>[4x]MASQTITVGPWGGPGGNEWDDGSYTGIRIIELSYKEAIGSFSVIYDLNGEPFSGSKHTSKLPYTNVKIELQFPEEFLVSVSGYTAPFSSLATRTPVVRSLKFKTNKGRTFGPYGEEDGTYFNLPIENGLVVGFKGRTGDLLDAIGVHMAL

Here, we report heterologous expression and production of soluble biologically active FTP in E. coli and also describe the crystal structure of Apo-FTP plus changes on binding α-D-glucose or α-D-mannose. The FTP structure showed a β-prism I fold, which is found in Jacalin, Artocarpin and other lectins giving a high structural similarity; except for a few loop areas around residues Leu90, Glu36 and Lys106, some of which are flexible and adopt different conformations, even in the same protein. Like most-known plant lectins, FTP is a hololectin defined as a multisubunit protein containing several carbohydrate-binding sites to allow cell agglutination. In contrast, FTP binds carbohydrates such as mannose and/or glucose in a different way, paralleling CMB and also Artocarpin presumably reflecting the high sequence identities of 90 and 91%, respectively.

Crystals of recombinant Apo-FTP grew in space group P212121 and diffracted to 1.55 Å at Diamond Light Source. Molecular replacement confirmed four monomers in the asymmetric unit and refinement gave a final model with Rfactor: 0.163 and Rfree: 0.200. All four monomers are almost identical and their superposition by α carbon (Cα) atoms gave an RMSD of ∼0.15 Å. However, the loops around Leu90, which are close to the carbohydrate-binding site, adopt different conformations in different subunits. Analysis using the PDB and PISA server suggests that FTP could be a dimer or tetramer in solution with stable interfaces between any of the two relative monomers. A total of 970 water molecules and 20 glycerol molecules were built into the electron density, with one glycerol molecule bound in the carbohydrate-binding site. Interestingly, in our Apo-FTP structure, there is a glycerol molecule (GOL18–a constituent of the crystallization condition) bound at the carbohydrate-binding site, forming two HBs bonds with the carboxylic side chain of Asp142 and one HB mediated by a water molecule with the carboxylic side chain of Asp139. There are three cis-prolines in each monomer all of which fit the electron density well, consistent with homologous structures of FTP.> PEKRLT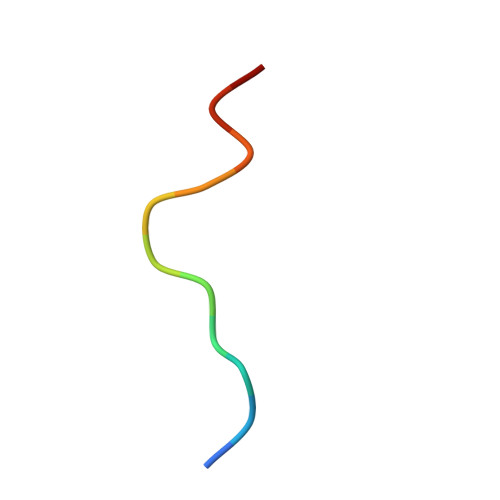VGSLRR> GSEFIKIRLTVLCAKNLAKKDFFRLPDPFAKIVVDGSGQCHSTDTVKNTLDPKWN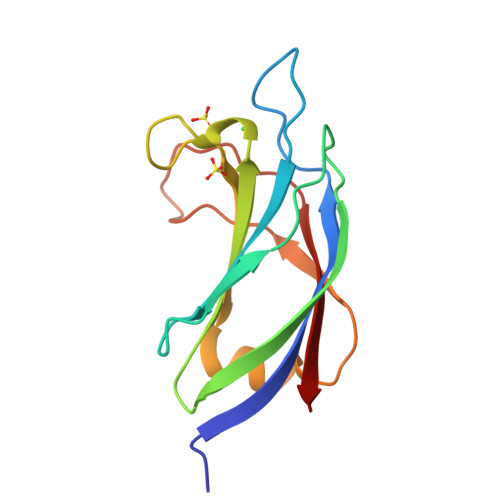QHYDLYVGKTDSITISVWNHKKIHKKQGAGFLGCVRLLSNAISRLKDTGYQRLDLCKLNPSDTDAVRGQIVVSLQTR> 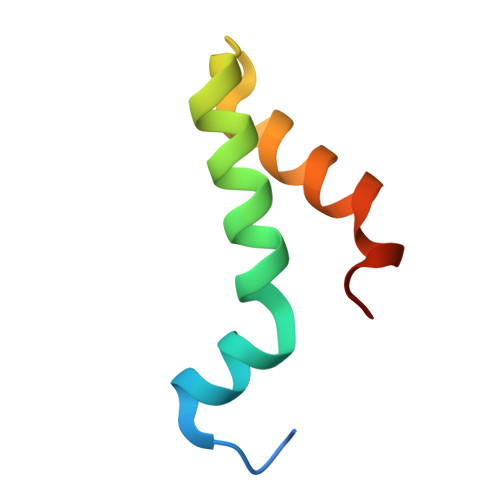GKVDLQSLPTRAYLDQTVVPILLQGLAVLAKERPPNPIEFLASYLLKNKAQFEDRN> MIIRDVELVKVARTPGDYPPPLKGEVAFVGRSNVGKSSLLNALFNRKIAFVSKTPGKTRSINFYLVNSKYYFVDLPGYGYAKVSKKERMLWKRLVEDYFKNRWSLQMV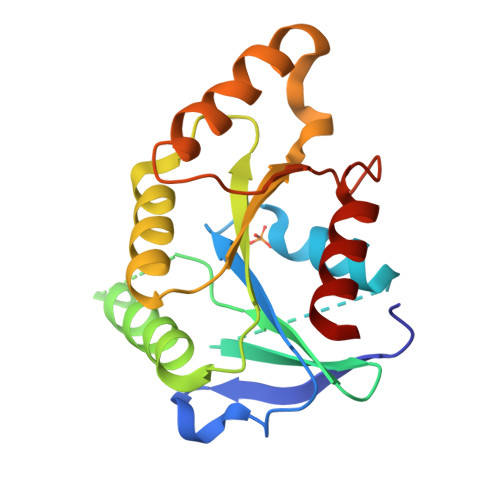FLLVDGRIPPQDSDLMMVEWMKSLNIPFTIVLTKMDKVKMSERAKKLEEHRKVFSKYGEYTIIPTSSVTGEGISELLDLISTLLKEN>GKLSEHLRYCDSILREMLSKKHAAYAWPFYKPVDAEALELHDYHDIIKHPMDLSTVKRKMDGREYPDAQGFAADVRLMFSNCYKYNPPDHEVVA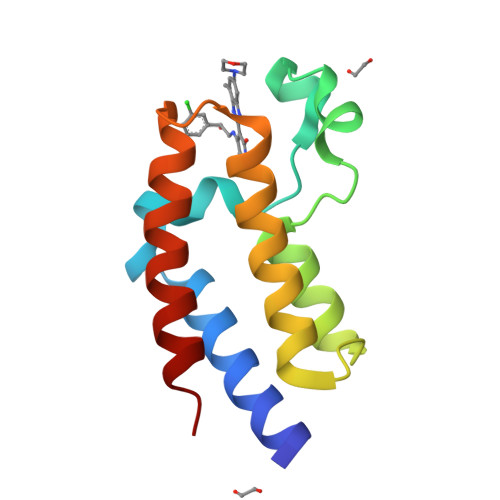MARKLQDVFEMRFAKMP[4x]> MNNNKA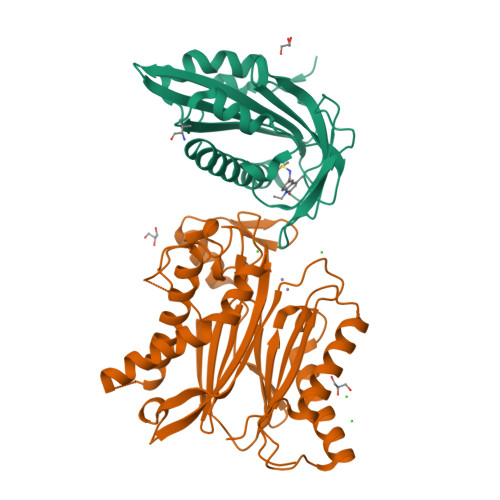EADTSSSMADPETRPTYTTHHLAIPSGVTQDEFDELKQSVVEFHTYQLSQNQCSSLLAQRIRAPNDVVWSIVRRFDQPQTYKHFIKSCSVSDNFTMAVGSTRDVNLISGLPAATSTERLDILDDDRQVLGISIIGGEHRLRNYRSVISVHGFNRDGAICTVALESYVVDVPEGNTEEDTRLFADTVVKLNLQKLVSVAESQVI;> RSVYELDCIPLWGTVSIQGNRSEMEDAFAVSPHFLKLPIKMLMGDHEGMSPSLTHLTGHFFGVYDGHGGHKVADYCRDRLHFALAEEIERIKDELCKRNTGEGRQVQWDKVFTSCFLTVDGEIEGKIGRAVVGSSDKVLEAVASETVGSTAVVALVCSSHIVVSNCGDSRAVLFRGKEAMPLSVDHKPDREDEYARIENAGGKVIQWQGARVFGVLAMSRSIGDRYLKPYVIPEPEVTFMPRSREDECLILASDGLWDVMNNQEVCEIARRRILMWHKKNGAPPLAERGKGIDPACQAAADYLSMLALQKGSKDNISIIVIDLKAQRKFKTRT>GHMATAPRPLREQYLHFQPISTRWHDNDIYGHVNNVTYYAFFDTAVNT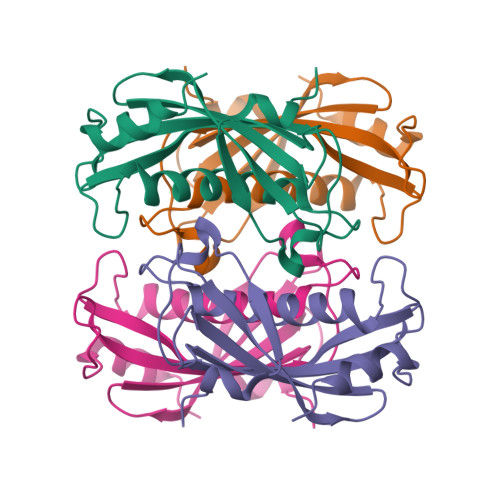YLIERGGLDIQGGEVIGLVVSSSCDYFAPVAFPQRIEMGLRVARLGNSSVQYELALFLEGQREACAAGRFVHVFVERRSSRPVAIPQELRDALAALQSSAQ[2x]> MEPGPTAAQRRCSLPPWLPLGLLLWSGLALGALPFGSSPHRVFHD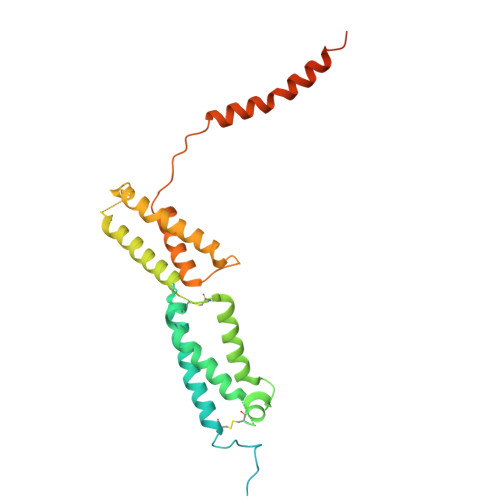LLSEQQLLEVEDLSLSLLQGGGLGPLSLPPDLPDLDPECRELLLDFANSSAELTGCLVRSARPVRLCQTCYPLFQQVVSKMDNISRAAGNTSESQSCARSLLMADRMQIVVILSEFFNTTWQEANCANCLTNNSEELSNSTVYFLNLFNHTLTCFEHNLQGNAHSLLQTKNYSEVCKNCREAYKTLSSLYSEMQKMNELENKAEPGTHLCIDVEDAMNITRKLWSRTFNCSVPCSDTVPVIAVSVFILFLPVVFYLSSFLHSEQKKRKLILPKRLKSSTSFANIQENSN> MSVIGVFSKGRATGHASVMSVLRYVPRARVPWQPSRFGRENLADDDMAQLWGTGRYRTGPGNYNSGYSTKKTHALEDSTVSIIPKHELEKFMPDISLGSKALVTPVSLMSARNGHRVTHDLIHSYDPYIGRLQKPAVVD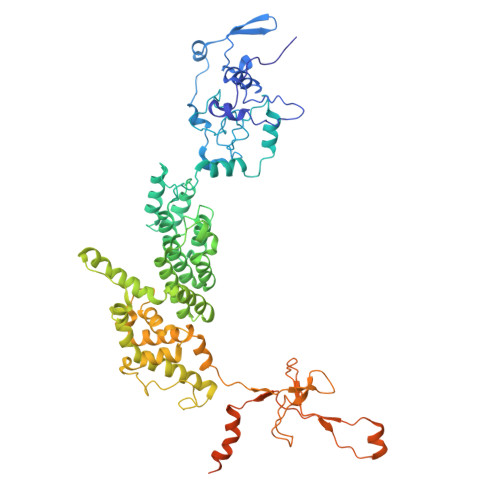HDNITVEDPNRVGLNAATLDCRSRIYRWLRRGPFFQEDNYFRRSTKLQRNGPVPVSVHEVPLMQRIIRLARRGHLKAACEEYRRVTSVPPVDVYRALTAACVPGAKLADAIAIFEDGHSRLFYVARDGEVLHNMLRCAIRAKHRVRVMWVYNVMVGRHYENVVVRAEVDVIWRYRIASLALEYLLDSNAGEEARTVYDYLVENELVDCDLHVRLGHVMQQALKEGKTVHVQQDALDGMALSQNVVAVAPQVAVAVYARYLETMQEGAAWTDARGLPLTDPAKTGADTNGAAAVAWLKAAFPDIDPVAVLRLARFRRSSKDLMAKDRPVYVQRAAQWVELLSSAHQTREEAPLTYLRKSRPSMANPNVRVAWLPERQRAHALLASDEGFKFAYAGPHTRFVEETFAYGENTLQSRYLAQQPVHTEVTPSVALGAAAVAAGMSSGSALPRLPGSSAAPQILHASVLLDGSLNGSSGSGTSTLRSGRNESAKAAASPTAGISSRPSSASSSAGLDDTHF> MAANKPKGQNSLALHKVIMVGSGGVGKSALTLQFMYDEFVEDYEPTKADSYRKKVVLDGEEVQIDILDTAGQEDYAAIRDNYFRSGEGFLCVFSITEMESFAATADFREQILRVKEDENVPFLLVGNKSDLEDKRQVSV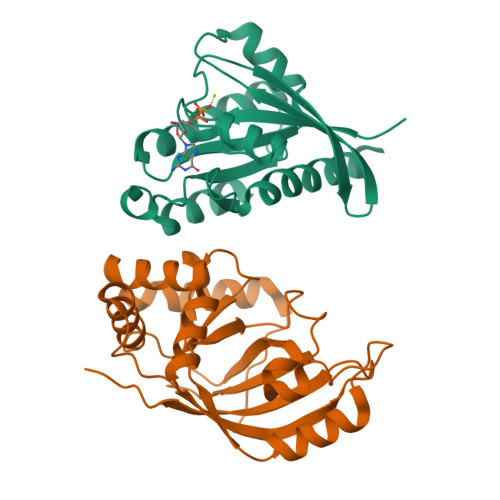EEAKNRAEQWNVNYVETSAKTRANVDKVFFDLMREIRARKMEDSKEKNGKKKRKSLAKRIRERCCIL;> MKGLRKSILCLVLSAGVIAPVTSGMIQSPQKCYAYSINQKAYSNTYQEFTNIDQAKAWGNAQYKKYGLSKSEKEAIVSYTKSASEINGKLRQNKGVINGFPSNLIKQVELLDKSFNKMKTPENIMLFRGDDPAYLGTEFQNTLLNSNGTINKTAFEKAKAKFLNKDRLEYGYISTSLMNVSQFAGRPIITKFKVAKGSKAGYIDPISAFAGQLEMLLPRHSTYHIDDMRLSSDGKQIIITATMMGTAINPK> MASPRSSGQPGPPPPPPPPPARLLL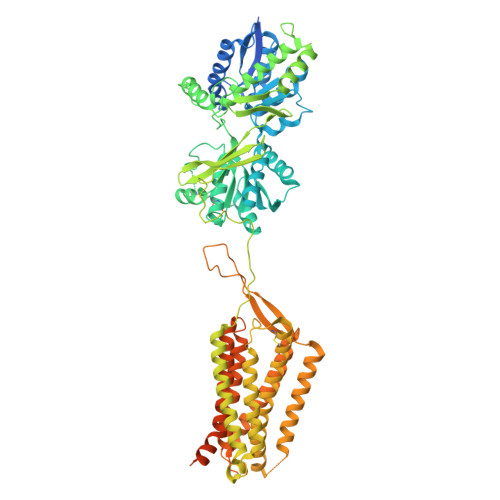LLLLPLLLPLAPGAWGWARGAPRPPPSSPPLSIMGLMPLTKEVAKGSIGRGVLPAVELAIEQIRNESLLRPYFLDLRLYDTECDNAKGLKAFYDAIKYGPNHLMVFGGVCPSVTSIIAESLQGWNLVQLSFAATTPVLADKKKYPYFFRTVPSDNAVNPAILKLLKHYQWKRVGTLTQDVQRFSEVRNDLTGVLYGEDIEISDTESFSNDPCTSVKKLKGNDVRIILGQFDQNMAAKVFCCAYEENMYGSKYQWIIPGWYEPSWWEQVHTEANSSRCLRKNLLAAMEGYIGVDFEPLSSKQIKTISGKTPQQYEREYNNKRSGVGPSKFHGYAYDGIWVIAKTLQRAMETLHASSRHQRIQDFNYTDHTLGRIILNAMNETNFFGVTGQVVFRNGERMGTIKFTQFQDSREVKVGEYNAVADTLEIINDTIRFQGSEPPKDKTIILEQLRKISLPLYSILSALTILGMIMASAFLFFNIKNRNQKLIKMSSPYMNNLIILGGMLSYASIFLFGLDGSFVSEKTFETLCTVRTWILTVGYTTAFGAMFAKTWRVHAIFKNVKMKKKIIKDQKLLVIVGGMLLIDLCILICWQAVDPLRRTVEKYSMEPDPAGRDISIRPLLEHCENTHMTIWLGIVYAYKGLLMLFGCFLAWETRNVSIPALNDSKYIGMSVYNVGIMCIIGAAVSFLTRDQPNVQFCIVALVIIFCSTITLCLVFVPKLITLRTNPDAATQNRRFQFTQNQKKEDSKTSTSVTSVNQASTSRLEGLQSENHRLRMKITELDKDLEEVTMQLQDTDYKDDDDK> CQGVA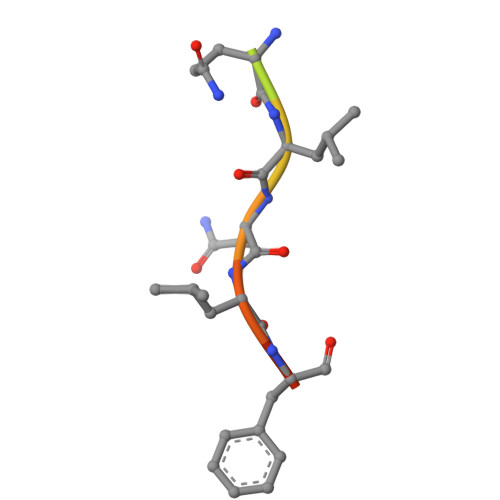QLNLFDD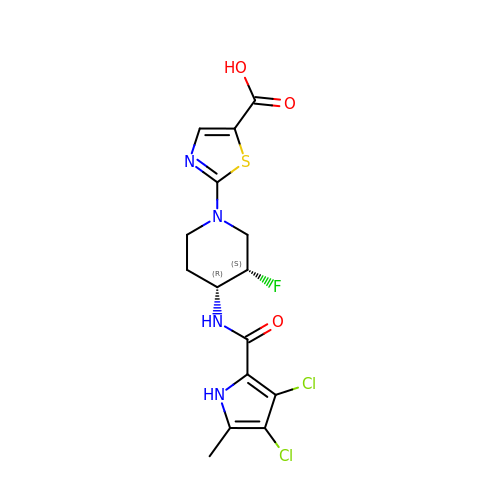2-[(3S,4R)-4-{[(3,4-dichloro-5-methyl-1H-pyrrol-2-yl)carbonyl]amino}-3-fluoropiperidin-1-yl]-1,3-thiazole-5-carboxylic acid | C15 H15 Cl2 F N4 O3 S | BGDGHNSKANYMHF-JGVFFNPUSA-N>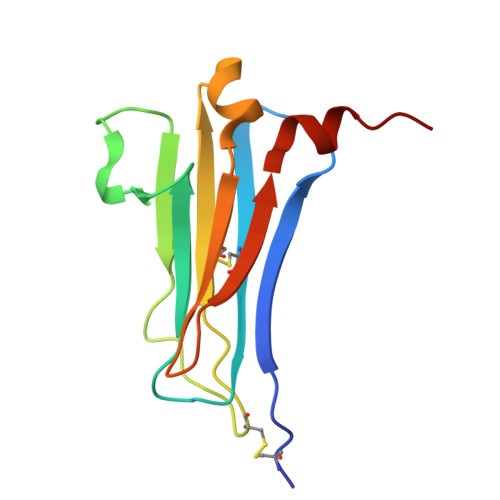 MECVKTRSVNIHVPVKETSKVVLECRGDSYFRHFSYVYWIIGKNKTVDQLPPNSGYRERIYLFKKPHRCENRPRADLILTNITDEMRNEKLTCVLIDPKDPLKESVILSKIWNCVYKI> PLPPLPPLP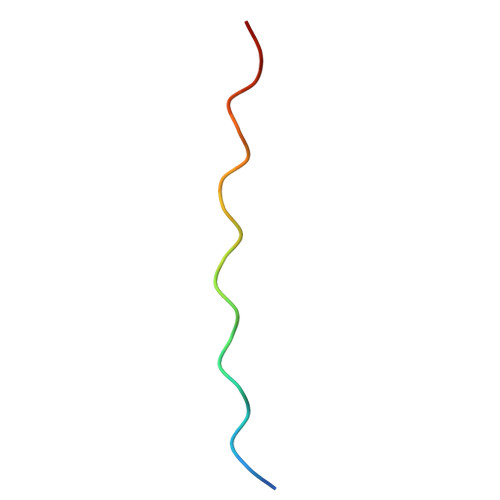PLPPLPPLPPLP>[2x]MLRSFVTSISPIGYNAVSLVSMRALATKAATTTTKKSTTKASPKTKKTTKKSTKPPKVDTKAIRLQKKINEARSAKKNLQQQIKDISTQHKTLSKQRKFEEKARSKIHKLAPGNFYSMFQKK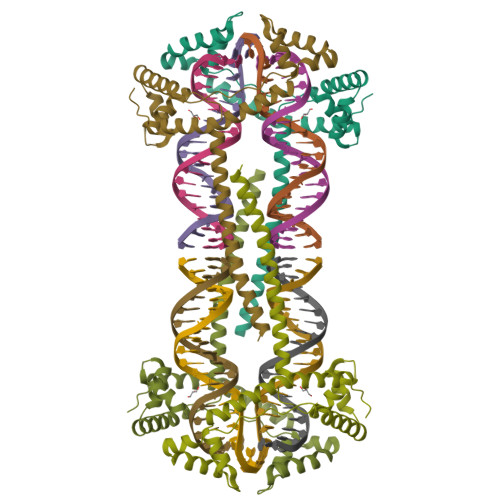RAGDSVAEFYQFPEEEKAKWIAARDAYWEKAKSYFTPKPKLGANGFAKYVQENYIRGDSLTETMKKLADEWNALSETEKQQYQISKEDKEKYKKALEKWKELRLKEYSDYLKFKENYKVEDDF> MKFTVEREHLLKPLQQVSGPLGGRPTLPILGNLLLQVADGTLSLTGTDLEMEMVARVALVQPHEPGATTVPARKFFDICRGLPEGAEIAVQLEGERMLVRSGRSRFSLSTLPAADFPNLDDWQSEVEFTLPQATMKRLIEATQFSMAHQDVRYYLNGMLFETEGEELRTVATDGHRLAVCSMPIG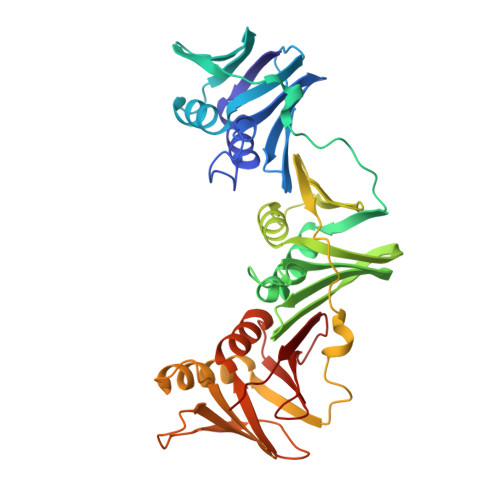QSLPSHSVIVPRKGVIELMRMLDGGDNPLRVQIGSNNIRAHVGDFIFTSKLVDGRFPDYRRVLPKNPDKHLEAGCDLLKQAFARAAAASNEKFRGVRLYVSENQLKITANNPEQEEAEEILDVTYSGAEMEIGFNVSYVLDVLNALKCENVRMMLTDSVSSVQIEDAASQSAAYVVMPMRL> SPASLASNLEISQSPTMPFW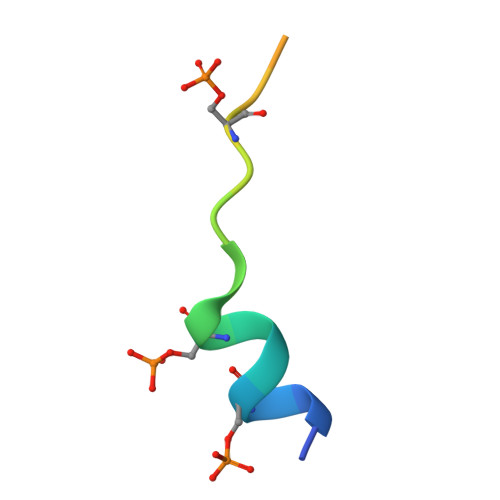S> GEFATSR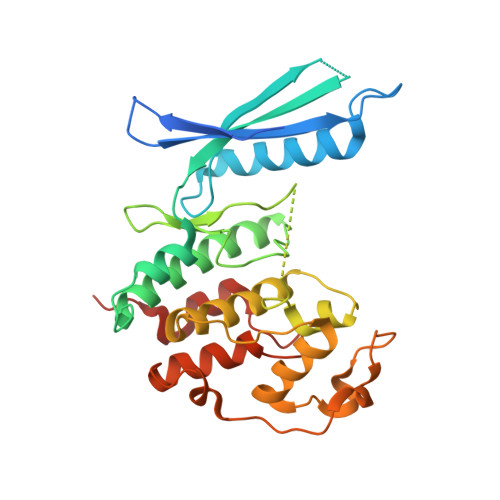YEPVAEIGVGAYGTVYKARDPHSGHFVALKSVRVPNGEEGLPISTVREVALLRRLEAFEHPNVVRLMDVCATSRTDREIKVTLVFEHVDQDLRTYLDKAPPPGLPAETIKDLMRQFLRGLDFLHANCIVHRDLKPENILVTSGGTVKLADFGLARIYSYQMALTPVVVTLWYRAPEVLLQSTYATPVDMWSVGCIFAEMFRRKPLFCGNSEADQLGKIFDLIGLPPEDDWPRDVSLPRGAFPPRGPRPVQSVVPEMEESGAQLLLEMLTFNPHKRISAFRALQHSYLHKDEGNPE> IEDSLCIAEGNNIDPFVSASTVQTGINIAGRILGVLGVPFAGQIASFYSFLVGELWPRGRDPWEIFLEHVEQLIRQQVTENTRDTALARLQGLGNSFRAYQQSLEDWLENRDDARTRSVLYTQYINLELDFLDAMPLFAIRNQEVPLLMVYAQAANLHLLLLRDASLFGSEFGLTSQEIQRYYERQVEKTREYSDYCARWYNTGLNNLRGTNAESWLRYNQFRRDLTLGVLDLVALFPSYDTRVYPMNTSAQLTREIYTDPIGRTNAPSGFASTNWFNNNAPSFSAIEAAVIRPPHLLDFPEQLTIFSVLSRWSNTQYMNYWVGHRLESRTIRGSLSTSTHGNTNTSINPVTLQFTSRDVYRTESFAGINILLTTPVNGVPWARFNWRNPLNSLRGSLLYTIGYTGVGTQLFDSETELPPETTERPNYESYSHRLSNIRLISGNTLRAPVYSWTHRSADRTNTISSDSITQIPLV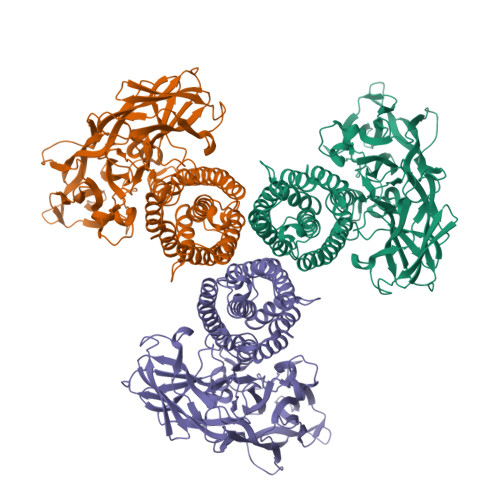KAHTLQSGTTVVKGPGFTGGDILRRTSGGPFAFSNVNLDFNLSQRYRARIRYASTTNLRIYVTVAGERIFAGQFDKTMDAGAPLTFQSFSYATINTAFTFPERSSSLTVGADTFSSGNEVYVDRFELIPVTATFEAESDLER> MAAAYLSRIQRGGHIQPFGCTLAVADDSSFRLLAFSEN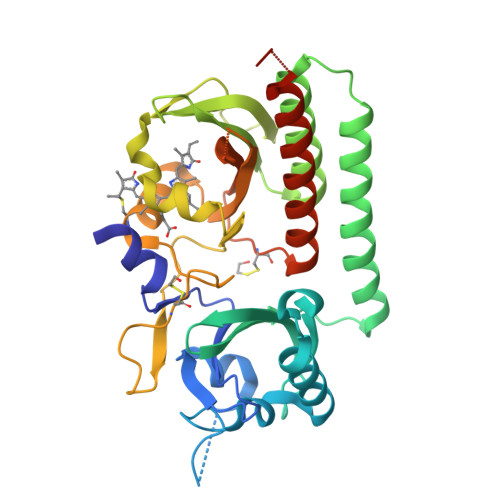AADLLDLSPHHSVPSLDSAAPPPVSLGADARLLFSPSSAVLLERAFAAREISLLNPLWIHSRVSSKPFYAILHRIDVGVVIDLEPARTEDPALSIAGAVQSQKLAVRAISRLQALPGGDIKLLCDTVVEHVRELTGYDRVMVYRFHEDEHGEVVAESRRDNLEPYLGLHYPATDIPQASRFLFRQNRVRMIADCHATPVRVIQDPGMSQPLCLVGSTLRAPHGCHAQYMANMGSIASLVMAVIISSGGDDEQTGRGGISSAMKLWGLVVCHHTSPRCIPFPLRYACEFLMQAFGLQLNMELQLAHQLSEKHHHHHH> MTVRKNQATLTADEKRRFVAAVLELKRSGRYDEFVRTHNEFIMSDTDSGERTGHRSPSFLPWHRRFLLDFEQALQSVDSSVTLPYWDWSADRTVRASLWAPDFLGGTGRSTDGRVMDGPFAASTGNWPINVRVDSRTYLRRSLGGSVAELPTRAEVESVLAISAY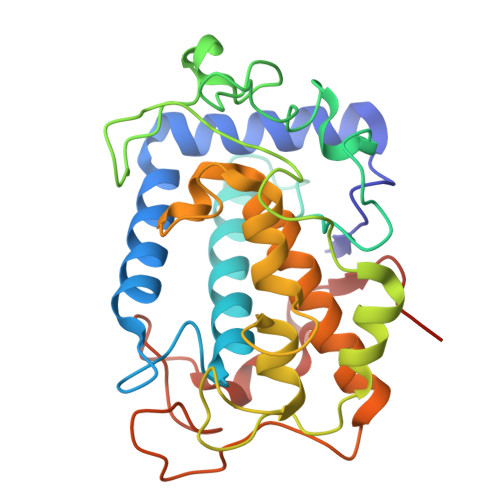DLPPYNSASEGFRNHLEGWRGVNLHNRVHVWVGGQMATGVSPNDPVFWLHHAYVDKLWAEWQRRHPDSAYVPTGGTPDVVDLNETMKPWNTVRPADLLDHTAYYTFDALEHHHHHH(2~{S})-2-[[(2~{S})-6-[[(2~{S})-2-[[4-[[[(2~{R})-2-[[(2~{R})-2-[(6-fluoranylpyridin-3-yl)carbonylamino]-5-oxidanyl-5-oxidanylidene-pentanoyl]amino]-5-oxidanyl-5-oxidanylidene-pentanoyl]amino]methyl]phenyl]carbonylamino]-3-naphthalen-2-yl-propanoyl]amino]-1-oxidanyl-1-oxidanylidene-hexan-2-yl]carbamoylamino]pentanedioic 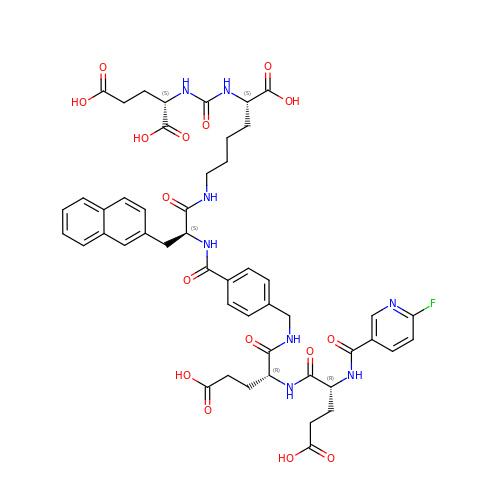acid | C49 H55 F N8 O16 | RFFFFGRYVZESLB-DWCHZDDLSA-N> MEKGDTHILVFPFPSQGAINPLLQLSKRLIAKGIKVSLVTTLHVSNHLQLQGAYSNSVKIEVISDGSEDRLETDTMRQTLDRFRQKMTKNLEDFLQKAMVSSNPPK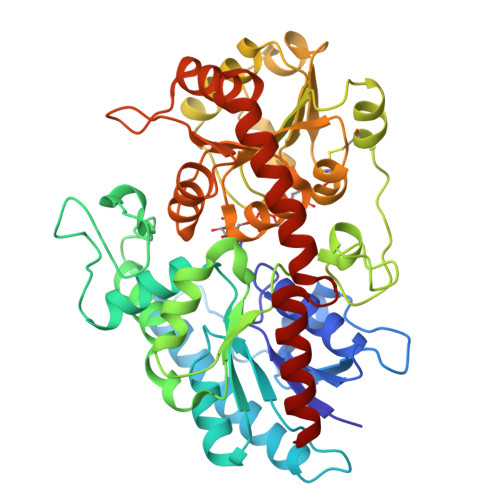FILYASTMPWVLEVAKEFGLDRAPFYTQSCALNSINYHVLHGQLKLPPETPTISLPSMPLLRPSDLPAYDFDPASTDTIIDLLTSQYSNIQDANLLFCNTFDKLEGEIIQWMETLGRPVKTVGPTVPSAYLDKRVENDKHYGLSLFKPNEDVCLKWLDSKPSGSVLYVSYGSLVEMGEEQLKELALGIKETGKFFLWVVRDTEAEKLPPNFVESVAEKGLVVSWCSQLEVLAHPSVGCFFTHCGWNSTLEALCLGVPVVAFPQWADQVTNAKFLEDVWKVGKRVKRNEQRLASKEEVRSCIWEVMEGERASEFKSNSMEWKKWAKEAVDEGGSSDKNIEEFVAMLKQT>MGLKALFFNVQGTLVDFYSTITREGEAFSAVRGFQADWTTVTEQWRAEYRSRLDQVIKGERPWTTTDRIYREALDGILANHPWGASLNSADRDELNSLWSKLIPWDDTAPGLARLRSKYITSTLSNGSMASVLRISKLGALPFDAILTAELVRSSKPDPKVYQLALDSVGIEAHQAMMVACHKYDLQAAKRLGFKVAFIARPFEFGPNKKVDTKPEQYFDYYANSVVELAGMLGALEHHHHHH[4x]

Microbial epoxide hydrolases, cis-epoxysuccinate hydrolases (CESHs), have been utilized for commercial production of enantiomerically pure L(+)- and D(−)-tartaric acids for decades. All these three CESH[L]s exhibit high sequence identity (>60%) with L-2-haloacid dehalogenases, which are members of the haloacid dehalogenase (HAD)-like superfamily. Studies have shown that both RhCESH[L] and KlCESH[L] adopt a two-step catalytic reaction mechanism by 18O-labeling studies.

We also constructed an inactive mutant, KlCESH[L]-D48N, to obtain the enzyme-substrate structure because D48 was proposed to be the first step catalytic residue. A product molecule, L-TA, was found in the substrate-binding site of KlCESH[L]-D48N, which was present in the crystallizing solutions at a concentration of 0.2 M. One carboxyl group of the L-TA is fixed by N165 and Y223, and the other carboxyl group is mainly fixed by the nitrogen atom of the main chain of V49 and Q50. The distances between the L-TA two hydroxyl oxygen atoms and the side chain oxygen atom of N48 are ∼2.5 to 3.0 Å, supporting that D48 is the nucleophilic residue in KlCESH[L]. However, D48 has similar distances to the two hydroxyl oxygen atoms of L-TA, making it difficult to determine which hydroxyl group is derived from the oxygen atom of the epoxy during the reaction. However, the binding of non-catalytic ligands, including sulfate ions and products L-TA, did not cause significant structural changes.(4R)-3-[(2S,3S)-3-[2-[4-[2-(dimethylamino)ethyl-methyl-amino]-2,6-dimethyl-phenoxy]ethanoylamino]-2-oxidanyl-4-phenyl-butanoyl]-5,5-dimethyl-N-[(1S,2R)-2-oxidanyl-2,3-dihydro-1H-inden-1-yl]-1,3-thiazolidine-4-carboxamide 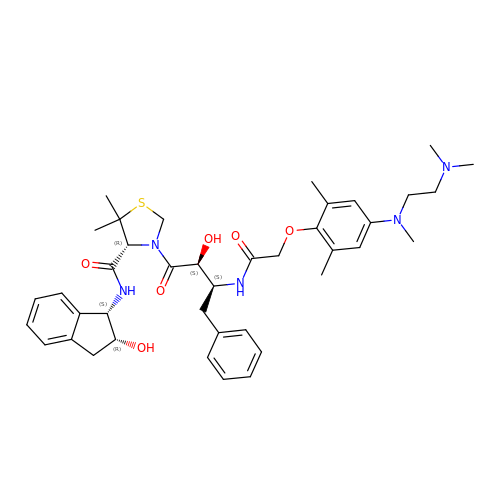| C40 H53 N5 O6 S | IZETWNQXMIHLNU-IVJJLKHCSA-N>[6x]MSRRPTLRLGLDRDVYNIVLNLEQQGTDENGKRPRLTVDYVYDTIKRSNSSLARQKKRMLEDSIERVLAVRKEQAKAEEETDSDDLIEAQERERERQKAAQAQRDANL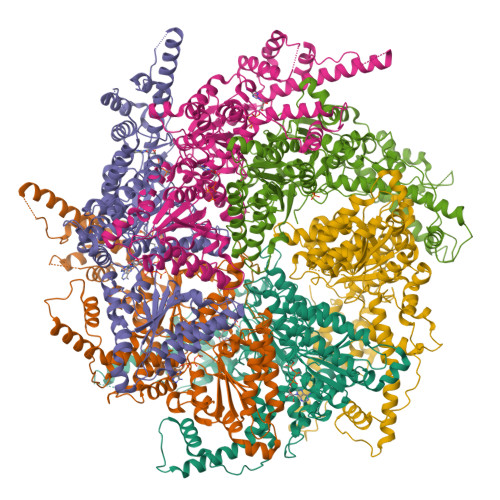LNRQIAKSWGFASSPGAKAADGEKGTDTGSIATPAPATPAVAENMAADTPTTSTGPVLPASSTDRQPNGEPRPKKRKAAPKEIDRTPPTKVSILDIAGVDDTLQRLLKEVWFPLRGGEACEKMGYRYDNGVLLHGPSGCGKTTLAHAIAGSIGVAFIPVSAPSVIGGTSGESEKNIRDVFDEAIRLAPCLIFLDEIDAIAGRRESANKGMESRIVAEIMNGMDRIRQNTPLGKNVVVLAATNRPEFLDPAIRRRFSVEIDMGMPSERAREQILRSLTRDLSLADDINFKELAKMTPGYVGSDLQYVVKAAVSESFQANIDSLLAQARAKHPADHLANVSQPQRDWLLLEAHRDEEVSWPSTKITMEQFRKAVSLVQPASKREGFSTIPDTTWSHVGALEDVRKKLEMSIIGPIKNPELFTRVGIKPAAGILLWGPPGCGKTLVAKAVANESKANFISIKGPELLNKYVGESERAVRQLFSRAKSSAPCILFFDQMDALVPRRDDSLSDASARVVNTLLTELDGVGDRSGIYVIGATNRPDMIDEAIRRPGRLGTSIYVGLPSAEDRVKILKTLYRNTVKAPKKREGTNGEDVDMTDAAAEQQHQGTTDADLEKVALDLRCTGFSGADLGNLMQAAAQACLERVYTQRQQKRKEGGSVAEEEEIEPVITMEDWEKALNEVKPSVKDPEKYMHSGFAAALEHHHHHH> GSTLVTGSEYETML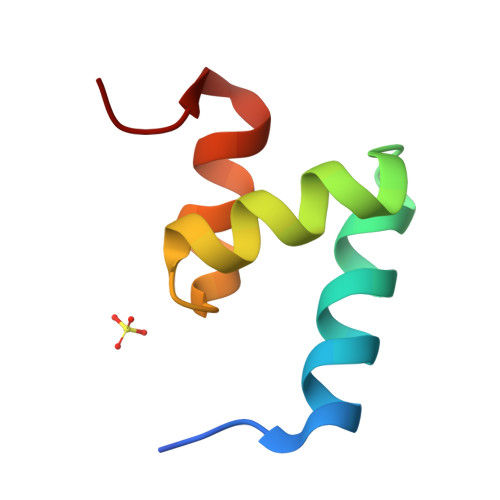TEIMSMGYERERVVAALRASYNNPHRAVEYLLTGIPG> DSVLLSGQTLYAGHSLTSGSYTLTIQNNCNLVKYQHGRQIWASDTDGQGSQCRLTLRSDGNLIIYDD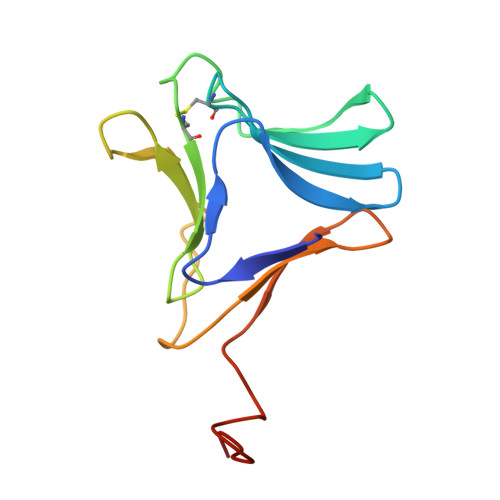NNMVVWGSDCWGNNGTYALVLQQDGLFVIYGPVLWPLGLNGCRSLN>MMNADMDAVDAEN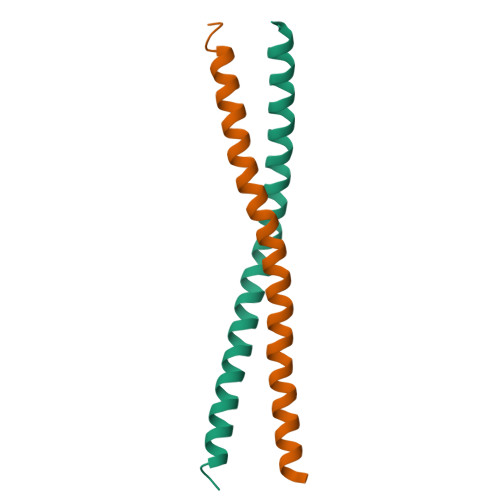QVELEEKTRLINQVMELQHTLEDLSARVDAVKEENLKLKSENQVLGQYIENLMSASSVFQTTDTKSKRK[3x]3,5-dioxo-4-(3-piperidin-1-ylpropyl)-2-[3-(trifluoromethyl)phenyl]-2,3,4,5-tetrahydro-1,2,4-triazine-6-carbonitrile 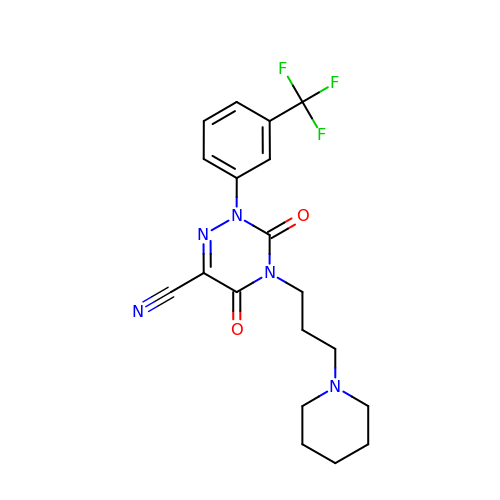| C19 H20 F3 N5 O2 | HKAVWQNLXOMWLR-UHFFFAOYSA-N DISTAMYCIN A | C22 H27 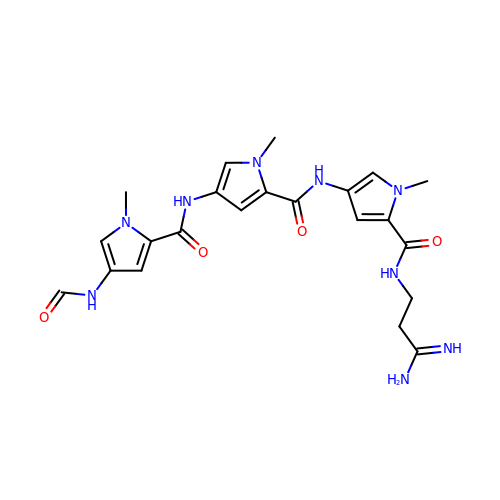N9 O4 | UPBAOYRENQEPJO-UHFFFAOYSA-N>MQPLVFDMAYENYMKRKELQNTVSQLLESEGWNRRNVDPFHIYFCNLKIDGALHRELVKRYQEKWDKLLLTSTEKSHVDLFPKDSIIYLTADSPNVMTTFRHDKVYVIGSFVDKSMQPGTSLAKAKRLNLATECLPLDKYLQWEIGNKNLTLDQMIRILLCLKNNGNWQEALQFVPK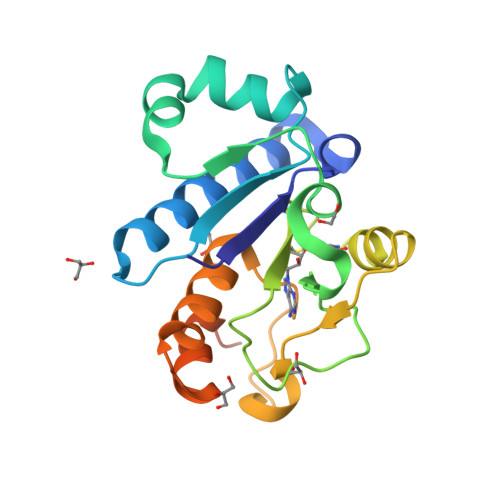RKHTGFLEISQHSQEFINRLKKAKT[3x]>MAGAIENARKEIKRISLEDHAESEYGAIYSVSGPVVIAENMIGCAMYELVKVGHDNLVGEVIRIDGDKATIQVYEETAGLTVGDPVLRTGKPLSVELGPGLMETIYDGIQRPLKAIKEESQSIYIPRGIDTPALDRTIKWQFTPGKFQVGDHISGGDIYGSVFENSLISSHKILLPPRSRGTITWIAPAGEYTLDEKILEVEFDGKKSDFTLYHTWPVRVPRPVTEKLSADYPLLTGQRVLDALFPCVQGGTTCIPGAFGCGKTVISQSLSKYSNSDAIIYVGCGERGNEMAEVLMEFPELYTEMSGTKEPIMKRTTLVANTSNMPVAAREASIYTGITLAEYFRDQGKNVSMIADSSSRWAEALREISGRLGEMPADQGFPAYLGAKLASFYERAGKAVALGSPDRTGSVSIVAAVSPAGGDFSDPVTTATLGITQVFWGLDKKLAQRKHFPSINTSVSYSKYTNVLNKFYDSNYPEFPVLRDRMKEILSNAEELEQVVQLVGKSALSDSDKITLDVATLIKEDFLQQNGYSTYDAFCPIWKTFDMMRAFISYHDEAQKAVANGANWSKLADSTGDVKHAVSSSKFFEPSRGEKEVHGEFEKLLSTMQERFAESTDDYKDHDGDYKDHDIDYKDDDDK[3x];>MVLSDKELFAINKKAVEQGFNVKPRLNYNTVSGVNGPLVILEKVKFPRYNEIVNLTLPDGTVRQGQVLEIRGDRAIVQVFEGTSGIDVKKTTVEFTGESLRIPVSEDMLGRIFDGSGRPIDNGPKVFAEDYLDINGSPINPYARIYPEEMISTGVSAIDTMNSIARGQKIPIFSASGLPHNEIAAQICRQAGLVRPTKDVHDGHEENFSIVFAAMGVNLETARFFKQDFEENGSLERTSLFLNLANDPTIERIITPRLALTTAEYLAYQTERHVLTILTDMSSYADALREVSAAREEVPGRRGYPGYMYTDLSTIYERAGRVEGRNGSITQIPILTMPNDDITHPIPDLTGYITEGQIFVDRQLHNKGIYPPINVLPSLSRLMKSAIGEGMTRKDHGDVSNQLYAKYAIGKDAAAMKAVVGEEALSIEDKLSLEFLEKFEKTFITQGAYEDRTVFESLDQAWSLLRIYPKEMLNRISPKILDEFYDRARDDADEDEEDPDTRSSGKKKDASQEESLI[3x];>MSSAITALTPNQVNDELNKMQAFIRKEAEEKAKEIQLKADQEYEIEKTNIVRNETNNIDGNFKSKLKKAMLSQQITKSTIANKMRLKVLSAREQSLDGIFEETKEKLSGIANNRDEYKPILQSLIVEALLKLLEPKAIVKALERDVDLIESMKDDIMREYGEKAQRAPLEEIVISNDYLNKDLVSGGVVVSNASDKIEINNTLEERLKLLSEEALPAIRLELYGPSKTRKFFD[3x];>MSQKNGIATLLQAEKEAHEIVSKARKYRQDKLKQAKTDAAKEIDSYKIQKD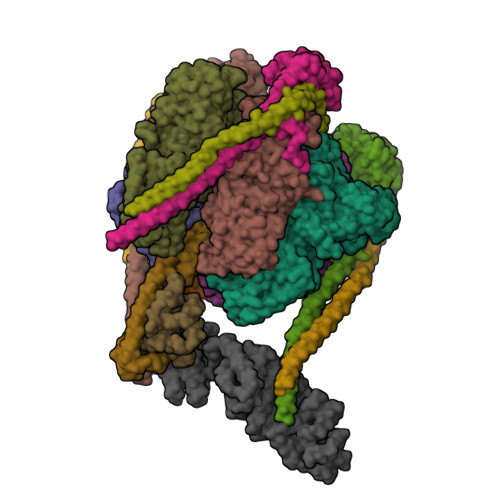KELKEFEQKNAGGVGELEKKAEAGVQGELAEIKKIAEKKKDDVVKILIETVIKPSAEVHINAL[3x];> MSGNREQVFPTRMTLGLMKTKLKGANQGYSLLKRKSEALTKRFRDITKRIDDAKQKMGRVMQTAAFSLAEVSYATGENIGYQVQESVSTARFKVRARQENVSGVYLSQFESYIDPEINDFRLTGLGRGGQQVQRAKEIYSRAVETLVELASLQTAFIILDEVIKVTNRRVNAIEHVIIPRTENTIAYINSELDELDREEFYRLKKVQEKKQNETAKLDAEMKLKRDRAEQDASEVAADEEPQGETLVADQEDDVIF;> MAEKRTLIAVIADEDTTTGLLLAGIGQITPETQEKNFFVYQEGKTTKEEITDKFNHFTEERDDIAILLINQHIAENIRARVDSFTNAFPAILEIPSKDHPYDPEKDSVLKRVRKLFGE;> MGATKILMDSTHFNEIRSIIRSRSVAWDALARSEELSEIDASTAKALESILVKKNIGDGLSSSNNAHSGFKVNGKTLIPLIHLLSTSDNEDCKKSVQNLIAELLSSDKYGDDTVKFFQEDPKQLEQLFDVSLKGDFQTVLISGFNVVSLLVQNGLHNVKLVEKLLKNNNLINILQNIEQMDTCYVCIRLLQELAVIPEYRDVIWLHEKKFMPTLFKILQRATDSQLATRIVATNSNHLGIQLQYHSLLLIWLLTFNPVFANELVQKYLSDFLDLLKLVKITIKEKVSRLCISIILQCCSTRVKQHKKVIKQLLLLGNALPTVQSLSERKYSDEELRQDISNLKEILENEYQELTSFDEYVAELDSKLLCWSPPHVDNGFWSDNIDEFKKDNYKIFRQLIELLQAKVRNGDVNAKQEKIIIQVALNDITHVVELLPESIDVLDKTGGKADIMELLNHSDSRVKYEALKATQAIIGYTFK{2-[(3S,4R)-3-(2-amino-6-oxo-1,6-dihydro-9H-purin-9-yl)-4-hydroxypyrrolidin-1-yl]-2-oxoethyl}phosphonic acid | C11 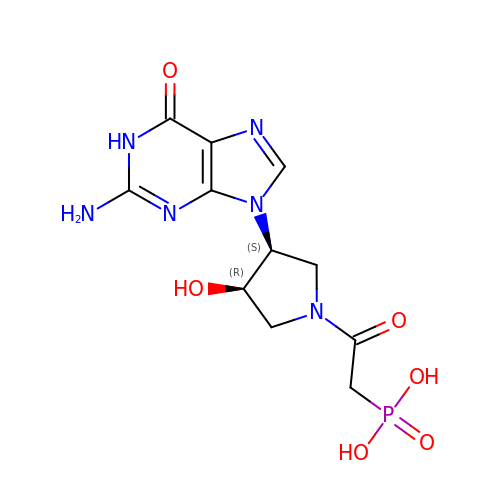H15 N6 O6 P | PIHCTBQWWHFPNB-NTSWFWBYSA-N> GAPEPHDSSHMDSEFRYTLFPIVYSIIFVLGVIANGYVLWVFARLYPCKK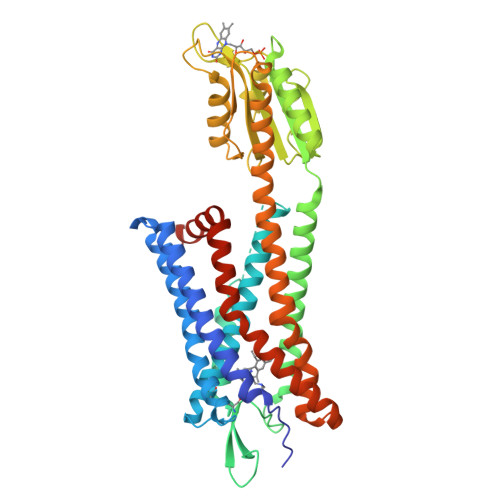FNEIKIFMVNLTMADMLFLITLPLWIVYYQNQGNWILPKFLCNVAGCLFFINTYCSVAFLGVITYNRYQAVTRPIKTAQANTRKRGISLSLVIWVAIVGAASYFLILDSTNTVPDSAGSGDVTRCFEHYEKGSVPVLIIHIFIVFSFFLVFLIILFCNLVIIRTLLMQAKALIVYGSTTGNTEYTAETIARELADAGYEVDSRDAASVEAGGLFEGFDLVLLGCSTWGDDSIELQDDFIPLFDSLEETGAQGRKVACFGCGDSSWEYFCGAVDAIEEKLKNLGAEIVQDGLRIDGDPRAARDDIVGWAHDVRGAIAEVKRRDLWMACTVLAVFIICFVPHHVVQLPWTLAELGFQDSKFHQAINDAHQVTLCLLSTNCVLNPVIYCFLTKKFRKHLTEKFYSMRSSRKEFLEVLFQ TAUROCHENODEOXYCHOLIC ACID | C26 H45 N O6 S | 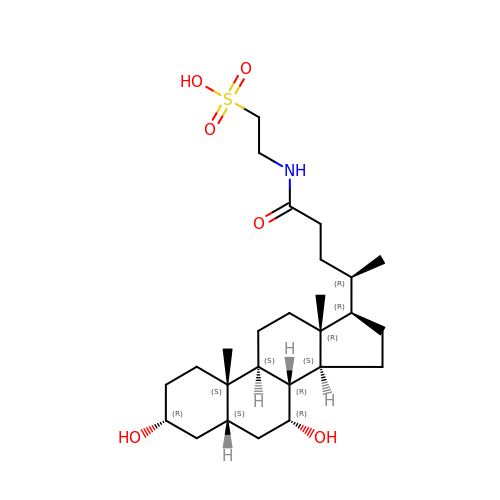BHTRKEVKTKCXOH-BJLOMENOSA-N> MDGAGAEEVLAPLRLAVRQQGDLVRKLKEDKAPQVDVDKAVAELKARKRVLEAKELALQPKDDIVDRAKMEDTLKRRFFYDQAFAIYGGVSGLYDFGPVGCALKNNIIQTWRQHFIQEEQILEIDCTMLTPEPVLKTSGHVDKFADFMVKDVKNGECFRADHLLKAHLQKLMSDKKCSVEKKSEMESVLAQLDNYGQQELADLFVNYNVKSPITGNDLSPPVSFNLMFKTFIGPGGNMPGYLRPETAQGIFLNFKRLLEFNQGKLPFAAAQIGNSFRNEISPRSGLIRVREFTMAEIEHFVDPSEKDHPKFQNVADLHLYLYSAKAQVSGQSARKMRLGDAVEQGVINNTVLGYFIGRIYLYLTKVGISPDKLRFRQHMENEMAHYACDCWDAESKTSYGWIEIVGCADRSCYDLSCHARATKVPLVAEKPLKEPKTVNVVQFEPSKGAIGKAYKKDAKLVMEYLAICDECYITEMEMLLNEKGEFTIETEGKTFQLTKDMINVKRFQKTLYVEEVVPNVIEPSFGLGRIMYTVFEHTFHVREGDEQRTFFSFPAVVAPFKCSVLPLSQNQEFMP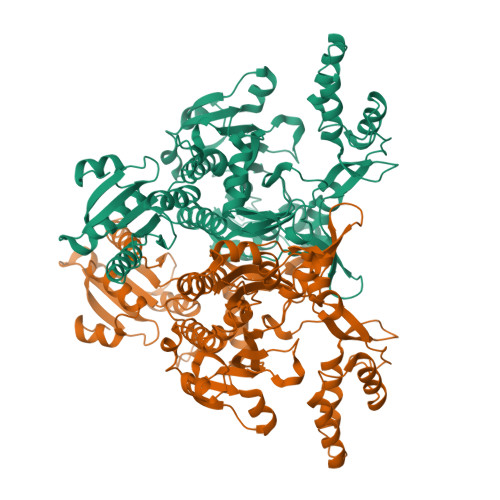FVKELSEALTRHGVSHKVDDSSGSIGRRYARTDEIGVAFGVTIDFDTVNKTPHTATLRDRDSMRQIRAEISELPSIVQDLANGNITWADVEARYPLFEGQETGKKETIEEHHHHHH> SAQTIEATSVKQLADAGVRVGDTLRISG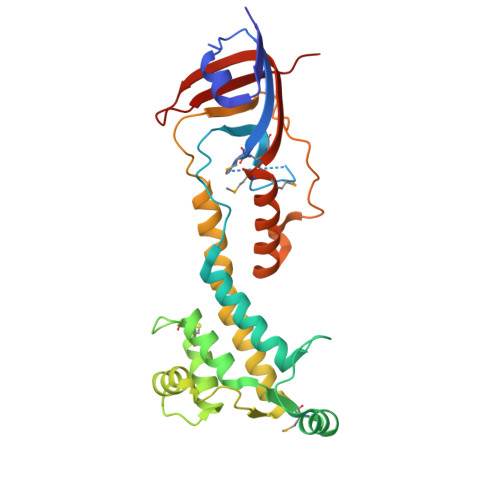TGMCNIRTSGTWSAKTNSPFLPFDCSQIIWNDARSLPLPESELVNKATALTEAVNRQLHPKPEDESRVSASLRSAIQKSGMVLLDDFGDIVLKTADLCSAKDDCVRLKNALVNLGNSKDWDALVKRANAGKLDGVNVLLRPVSAESLDNLVATSTAPFITHETARAAQSLNSPAPGGFLIVSDEGSDFVDQPWPSASLYDYPPQEQWNAFQKLAQMLMHTPFNAEGIVTKIFTDANGTQHIGLHPIP ErmE (EC 2.1.1.184) is a dimethyltransferase from the actinomycete Saccharopolyspora erythraea, from which the first macrolide antibiotic erythromycin was originally extracted. ErmE provides resistance to macrolide, lincosamide, and streptogramin B (MLS) antibiotics to S. erythraea. The bilobed structure of ErmE consists of an N-terminal Rossmann-like α/ß catalytic domain (residues 42–211) and C-terminal helical domain (residues 219–285), which are connected by a loop.

Here, we present the first crystal structure of rRNA methyltransferase ErmE, determined at 1.75-Å resolution. Only the truncated version of ErmE produced diffraction-quality crystals. The refined structure includes residues 42–285 of ErmE. The absence of ordered density for the N- and C-termini confirms the predicted flexibility of these regions. SEC analysis and examination of the structure in PDBe PISA33 confirm that ErmE is a monomer. The N-terminal domain shows an L-shaped pocket rich in conserved residues. Superposition of the catalytic domains of ErmE and ErmC’ in complex with SAM suggests that SAM will bind similarly in the lower part of the pocket, with the methyl group directed towards the upper part of the pocket, where the substrate adenine will likely bind. Interestingly, the substitution of Asn101 in ErmC’ with Ala131 in ErmE suggests that the carboxyl group of SAM will only be coordinated through a hydrogen bond to the main chain N of Leu44, while in ErmC’ the same carboxyl in addition hydrogen bond to Asn101 Nδ2. In the ErmE structure, a sulfate ion is bound between Lys164 and Arg174, possibly mimicking a substrate phosphate.

> MHHHHHHHHMSSSDEQPRPRRRNQDRQHPNQNRPVLGRTERDRNRRQFGQNFLRDRKTIARIAETAELRPDLPVLEAGPGEGLLTRELADRARQVTSYEIDPRLAKSLREKLSGHPNIEVVNADFLTAEPPPEPFAFVGAIPYGITSAIVDWCLEAPTIETATMVTQLEFARKRTGDYGRWSRLTVMTWPLFEWEFVEKVDRRLFKPVPKVDSAIMRLRRRAEPLLEGAALERYESMVELCFTGVGGNIQASLLRKYPRRRVEAALDHAGVGGGAVVAYVRPEQWLRLFERLDQKNEPRLE> MFKDFFNRTKKKKYLTVQDSKNNDVPAGIMTKCPKCKKIMYTKELAENLNVCFNCDHHIALTAYKRIEAISDEGSFTEFDKGMTSANPLDFPSYLEKIEKDQQKTGLKEAVVTGTAQLDGMKFGVAVMDSRFRM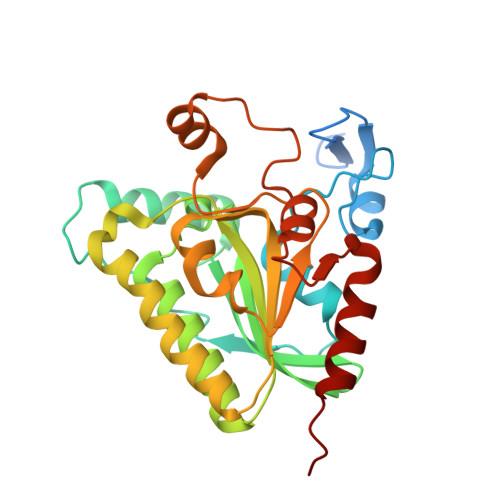GSMGSVIGEKICRIIDYCTENRLPFILFSASGGARMQEGIISLMQMGKTSVSLKRHSDAGLLYISYLTHPTTGGVSASFASVGDINLSEPKALIGFAGRRVIEQTINEKLPDDFQTAEFLLEHGQLDKVVHRNDMRQTLSEILKIHQEVTK> PAARVEYIAPWWVVWLHSVPHLGLRLQRVDSTFSPGDETYQESLLFLGVLAAIGLGLNLIFLTVYLVCTCCCRRDHTVQTKQQESCCVTWTAVVAGLLCCAAVGVGFYGNSETNDGMHQLIYSLDNANHTFSGMDELVSANTQRMKVDLEQHLARLSEIIAARGDYIQTLKFMQQMAGNVVSQLSGLPVWREVTTQLTKLSHQTAYVEYYRWLSYLLLFILDLVICLVTCLGLARRSKCLLASMLCCGILTLILSWASLAADAAAAVGTSDFCMAPDIYILNNTGSQINSEVTRYYLHCSQSLISPFQQSLTTFQRSLTTMQIQVGGLLQFAVPLFPTAEKDLLGIQLLLNNSEISLHQLTAMLDCRGLHKDYLDALTGICYDGIEGLLFLGLFSLLAALAFSTLTCAGPRAWKYFINRDRDYDDIDDDDPFNPQARRIAAHNPTRGQLHSFCSYSSGLGSQCSLQPPSQTISNAPVSEYMNQAILFGGNPRYENVPLIGRGS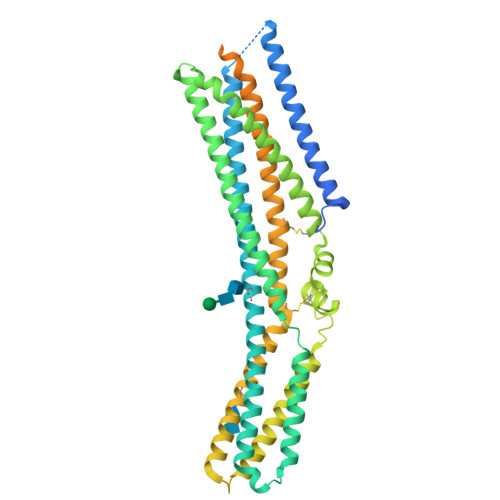PPPTYSPSMRPTYMSVADEHLRHYEFPSSNSLEVLFQ>MALRADQVSLIGQVFESYLLQHHRDDILGILRQGDDEAHYPVLVDALTLFETNMEIGEYFNAFPSQVLPIFDGALRRAAMAVLQAATPSPELRMKPNLHARISGLPICPELTREHIPKTRDVGHFLSVTGTVIRTSLVKVLEFERSYICNKCKHVFVAKADFEQYYAFCRPSACLNEEGCNSTKFTCLSGTSSSPSSCRDYQEIKIQEQVQRLSVGSIPRCMVVVLEDDLVDSCKSGDDITVYGVVMQRWKPFHQDARCDLELVLKANYVKVN[3x];>ASSRLVQSTLDQFIPYKGWKLYFSEAYADKSPFVQKTQAFEKFFMQRIELYDKDEIERKGSILVDYKELIEDRELTKSIPNISTELRDMPQKILQCMGLAIHQVLTKDLERHAAELQVQEGLPLDGEPIINVPLIHARLYNYEPLTQLKNVRANCYGKYIALRGTVVRVSNIKPLCTKLAFVCGTCGDVQSVPLPDGKYTLPTKCLVPECRGRSFTPDRSSPLTATVDWQSVKVQELMSDDQREAGRIPRTIECELVQDLVDSCVPGDVVTITGVVKVSSTEEGASKNKNDKCVFLLYIEANSVSNSK[3x]

MCM8 and MCM9 form a functional helicase complex (MCM8/9) that plays an essential role in DNA homologous recombination repair for DNA double-strand break. MCM8 and MCM9 proteins are structurally similar, with an MCM domain at the N-terminus (NTD) and an AAA+ ATPase domain at the C-terminus (CTD). The structures reveal that MCM8/9 is arranged into a heterohexamer through a threefold symmetry axis, creating a central channel that accommodates DNA. Multiple characteristic hairpins from the N-terminal oligosaccharide/oligonucleotide (OB) domains of MCM8/9 protrude into the central channel and serve to unwind the duplex DNA.

As our previous study shows the hMCM8/9 helicase complex is unstable for high-resolution structure determination, we first solved the cryo-EM structure of the MCM8/9 complex from Gallus gallus. Based on the electron density map, the structures of the NTD and CTD were reconstructed at the resolutions of 3.66 Å and 5.21 Å, respectively, and then aligned into a composite structure. The structure reveals that gMCM8 and gMCM9 alternately assemble into a pinwheel-like hexamer with a central channel. The assembly pattern of the gMCM8/9 complex with a threefold (C3) symmetry axis is unique among MCM helicases. In addition, a distinguishing feature of the gMCM8/9 is that the helical domain of gMCM8 contains a long α5 helix that protrudes around the hexameric ring. The dimer interface between NTDs of gMCM8 and gMCM9 is largely composed of the β-strands from the OB domain of gMCM9 and the flanking ZF and OB domain of gMCM8. Compared to the strong interaction between the dimer interface, the interaction within the trimer interface is weaker. The trimer interface is dominated by electrostatic interaction and hydrogen-bonding interactions. Based on the preceding analysis, we assume that opening a ‘gate’ on the trimer interface for DNA loading will be easier than on the dimer interface. Therefore, we presume the current structure of gMCM8/9 may represent a loading state of MCM8/9 helicase.> SRVSVTDYKRLLDSGAFHLLLDVRPQVEVDICRLPHALHIPLKHLERRDAESLKLLKEAIWEEKQGTQEGAAVPIYVICKLGNDSQKAVKILQSLSAAQELDPL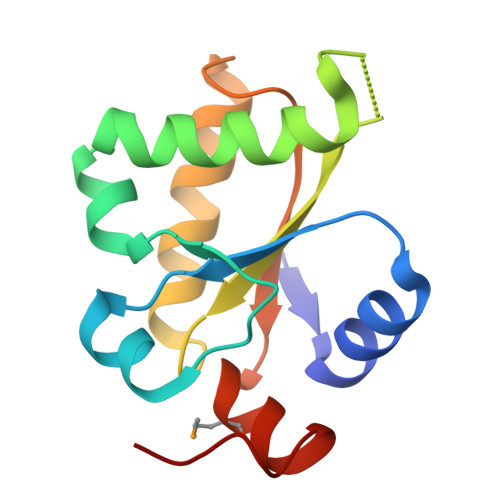TVRDVVGGLMAWAAKIDGTFPQY> KFDVNTSAVQVLIEHIGNLDRAYEFAERCNEPAVWSQLAKAQLQKGMVKEAIDSYIKADDPSSYMEVVQAANTSGNWEELVKYLQMARKKARESYVETELIFALAKTNRLAELEEFINGPNNAHIQQVGDRCYDEKMYDAAKLLYNNVSNFGRLAST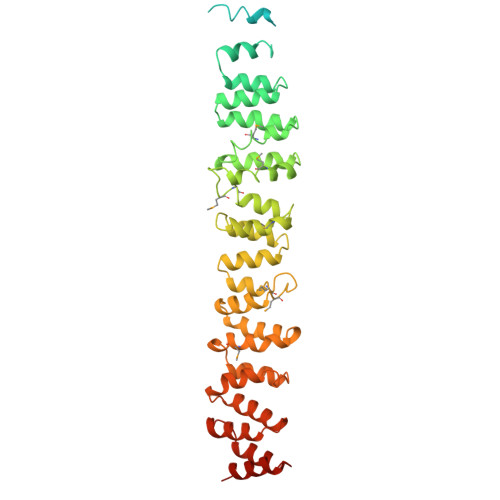LVHLGEYQAAVDGARKANSTRTWKEVCFACVDGKEFRLAQMCGLHIVVHADELEELINYYQDRGYFEELITMLEAALGLERAHMGMFTELAILYSKFKPQKMREHLELFWSRVNIPKVLRAAEQAHLWAELVFLYDKYEEYDNAIITMMNHPTDAWKEGQFKDIITKVANVELYYRAIQFYLEFKPLLLNDLLMVLSPRLDHTRAVNYFSKVKQLPLVKPYLRSVQNHNNKSVNESLNNLFITEEDYQALRTSIDAYDNFDNISLAQRLEKHELIEFRRIAAYLFKGNNRWK>[2x]KKPLFTKSPRNSASCESTITLQSNLLFTYYKHYFAGIKKVALIGFPDHPNKGDSAIYVAEKKLLDALNIEVVYITAQEADYSASELKSIISDIPRDEFALAFHGGGNFGDLYPDHQHLRELVVRDFPSFTTISFPQSVWYNEQQLLEQASILYAENPNITLVTRDRQSYGFAVDAFGKHNEVLLTPDIVFFMGPIPEIREATPITHDVLILARLDHEGGQQHGAEDYYRDTLN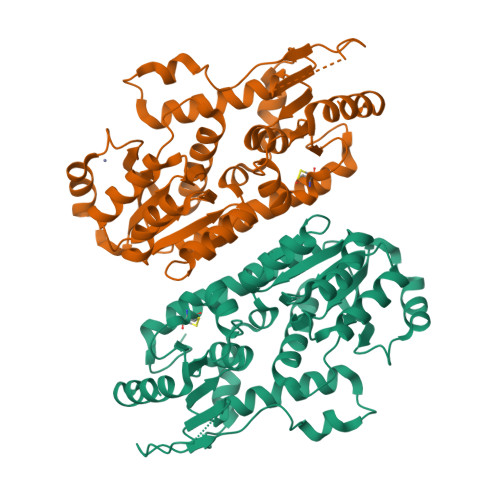AANLTYSVEDWLLWDPPVAQNPDSSFDDRGQARYEAGAEFLASARVVITDRLHAHILSTLMGIPHIVVENSQMGKITNYHNTWLHGCTLDGVSVVVDSVDKALSLLLEWNEAGYF> MDGAGAEEVLAPLRLAVRQQGDLVRKLKEDKAPQVDVDKAVAELKARKRVLEAKELALQPKDDIVDRAKMEDTLKRRFFYDQAFAIYGGVSGLYDFGPVGCALKNNIIQTWRQHFIQEEQILEIDCTMLTPEPVLKTSGHVDKFADFMVKDVKNGECFRADHLLKAHLQKLMSDKKCSVEKKSEMESVLAQLDNYGQQELADLFVNYNVKSPITGNDLSPPVSFNLMFKTFIGPGGNMPGYLRPETAQGIFLNFKRLLEFNQGKLPFAAAQIGNSFRNEISPRSGLIRVREFTMAEIEHFVDPSEKDHPKFQNVADLHLYLYSAKAQVSGQSARKMRLGDAVEQGVINNTVLGYFIGRIYLYLTKVGISPDKLRFRQHMENEMAHYACDCWDAESKTSYGWIEIVGCADRSCYDLSCHARATKVPLVAEKPLKEPKTVNVVQFEPSKGAIGKAYKKDAKLVMEYLAICDECYITEMEMLLNEKGEFTIETEGKTFQLTKDMINVKRFQKTLYVEEVVPNVIEPSFRLGRIMYTVFEHTFHVREGDEQRTFFSFPAVVAPFKCSVLPLSQNQEFMPFVKELSEALTRHGVSHKVDDSSGSIGRRYARTDEIGVAFGVTIDFDTVNKTPHTATLR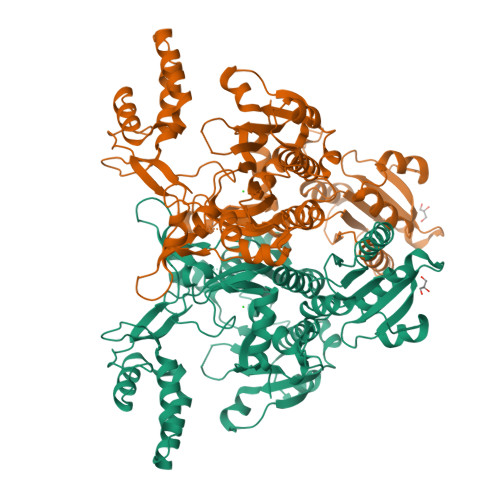DRDSMRQIRAEISELPSIVQDLANGNITWADVEARYPLFEGQETGKKETIEELEHHHHHH PDFs are ubiquitous essential metalloenzymes which co-translationally remove the formyl group carried by the initiator methionine in bacteria, mitochondria and chloroplast. Here, we present and characterize a PDF enzyme issued from the bacterium Streptococcus agalactiae (SaPDF) which behaves as an excellent structural platform to describe PDF-inhibitor interactions. Like most other PDFs, SaPDF behaves as a monomer and its crystal structure reveals a classical PDF fold. In addition, SaPDF contains the typical insertions of type 2 PDFs12, including an eight-amino acids loop folded as an α-helix (insertion 2) and a long loop connecting strands β2 and β3 usually referred as the CD-loop (insertion 3).

The apo-protein crystallized in two different crystallization conditions, which gave highly similar structures (root mean square deviation between all Cα is 0.307 Å). According to this measure, both free SaPDF crystallized in a slightly open conformation (δap measured between C131, H178 and V71 is respectively 48.0° and 47.5°). Like other PDFs10, the core of SaPDF is composed of two α-helices, three 310-helices and eight β-strands organized in two β-sheets. The structure is organized into two sub-domains around the active site, called N- and C-terminal sub-domains.

> MAAIDKLVKASHLIDMNDIIREGNPTLRKVAEEVTFPLSEKEEILGEKMMQFLKHSQDPIMAEKLGLRGGVGLAAPQLDISKRIIAVLVPNVEDAQGNPPKEAYSLQEVMYNPKVVSHSVQDAALSDGEGCLSVDREVPGYVVRHARVTIEYFDKTGEKHRLKLKGYNSIVVQHEIDHIDGIMFYDRINEKNPFAVKEGLLILE>[2x]MHHHHHHGSMSMPNHQNMLDNQTILITGGTGSFGKCFVRKVLDTTNAKKIIVYSRDELKQSEMAMEFNDPRMRFFIGDVRDLERLNYALEGVDICIHAAALKHVPIAEYNPLECIKTNIMGASNVINACLKNAISQVIALSTDKAANPINLYGATKLCSDKLFVSANNFKGSSQTQFSVVRYGNVVGSR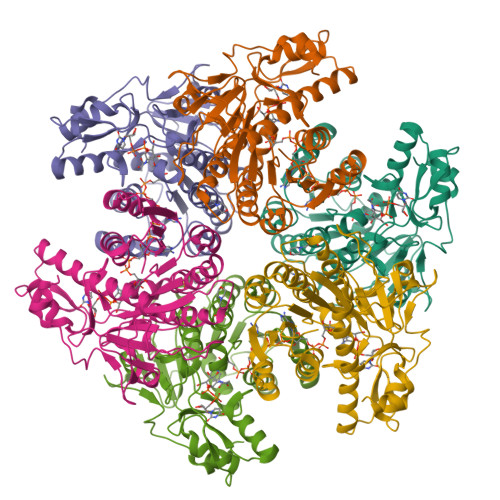GSVVPFFKKLVQNKASEIPITDIRMTRFWITLDEGVSFVLKSLKRMHGGEIFVPKIPSMKMTDLAKALAPNTPTKIIGIRPGEKLHEVMIPKDESHLALEFEDFFIIQPTISFQTPKDYTLTKLHEKGQKVAPDFEYSSHNNNQWLEPDDLLKLL> MEYQHWLREAISQLQASESPRRDAEILLEH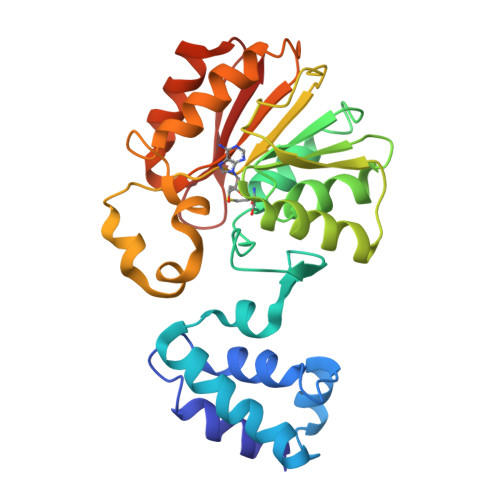VTGRGRTFILAFGETQLTDEQCQQLDALLTRRRDGEPIAHLTGVREFWSLPLFVSPATLIPRPDTECLVEQALARLPEQPCRILDLGTGTGAIALALASERPDCEIIAVDRMPDAVSLAQRNAQHLAIKNIHILQSDWFSALAGQQFAMIVSNPPYIDEQDPHLQQGDVRFEPLTALVAADSGMADIVHIIEQSRNALVSGGFLLLEHGWQQGEAVRQAFILAGYHDVETCRDYGDNERVTLGRYYQ>[2x]KDIIELTDTYGANNYHPLPIVISKAEGVWVEDPEGNRYMDLLSAYSAVNQGHRHPKIINALIDQANRVTLTSRAFHSDQLGPWYEKVAKLTNKEMVLPMNTGAEAVETAIKTARRWAYDVKKVEANRAEIIVCEDNFHGRTMGAVSMSSNEEYKRGFGPMLPGIIVIPYGDLEA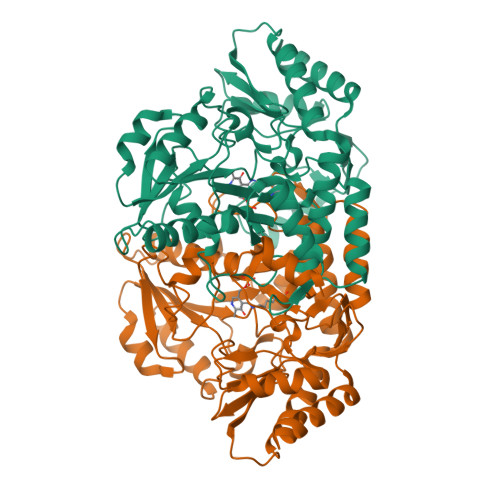LKAAITPNTAAFILEPIQGEAGINIPPAGFLKEALEVCKKENVLFVADEIQTGLGRTGKVFACDWDNVTPDMYILGKALGGGVFPISCAAANRDILGVFEPGSHGSTFGGNPLACAVSIAALEVLEEEKLTERSLQLGEKLVGQLKEIDNPMITEVRGKGLFIGIELNEPARPYCEQLKAAGLLCKETHENVIRIAPPLVISEEDLEWAFQKIKAVLS1-{2-OXO-3-[(1R)-1-(1H-PYRROL-2-YL)ETHYL]-2H-INDOL-5-YL}UREA 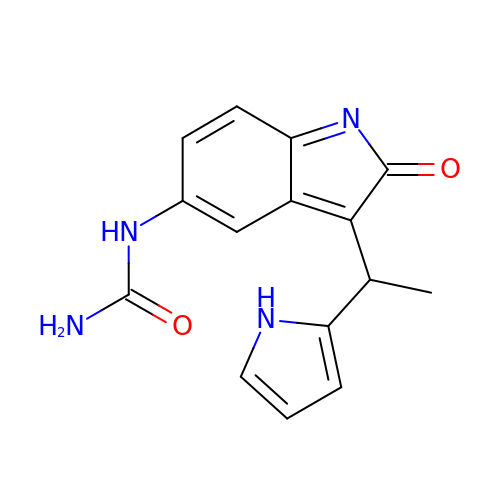| C15 H14 N4 O2 | KJDBLWKTHMHALD-QMMMGPOBSA-N> GSTGSPPGPPGVVIVEEITESTATLSWSPATDNHSPISSYNLQARSPFSLGWQTVKTVPEVITGDMESAMAVDLNPWVEYEFRVVATNPIGTGDPSIPSRMIRTNEAVPKTAPSNVSGRSGRRHELVIAWEPVSEEFQNGEGFGYIVAFRPNGTRGWKEKMVTSSEASKFIYRDESVPPLTPFEVKVGVYNNKGDGPFSQIVVICSAEGEPTAAPTDVTATSVSVSEIFVVWKHVKESLGRPQGFEISYWKDTEPE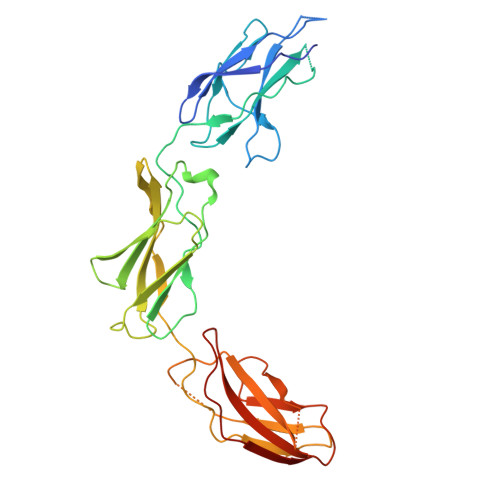DSVETVRTRGNESFVMLTGLEGNTLYHLTVRAYNGAGYGPPSREASTTTKR[(5-{4-fluoro-2-[2-(1H-imidazol-1-yl)ethoxy]phenyl}-1H-indazol-3-yl)methyl]dimethylamine | C21 H22 F N5 O | 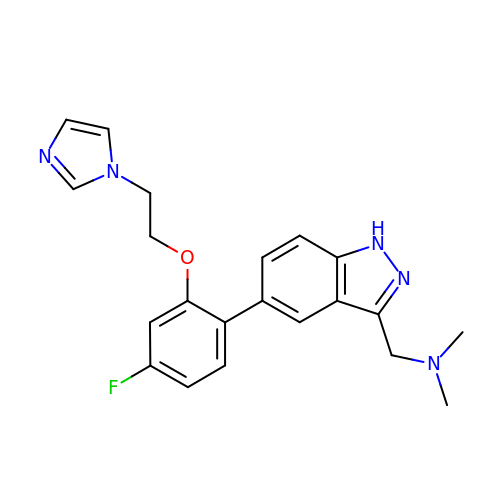YRWJVRAKMIULHA-UHFFFAOYSA-N>AASEDEFLRYLWRDYLYPKQYAWVLIAAYVAVFVVALVGNTLVCLAVWRNHHMRTVTNYFLVNLSLADVLATAICLPASLLVDITESWLFGHALCKVIPYLQAVSVSVAVLTLSFIALDRWYAICHPLLFKSTARRALGSILGIWAVSLAIMVPQAAVMECSSVLPELAARTRAFSVCDERWADDLAPKIYHSCFFIVTYLAPLGLMAMAYFQIFRKLWGRQIPGTTSALVRNWKRPSDQLGDLEQGLSGEPQPRARAFLAEVKQ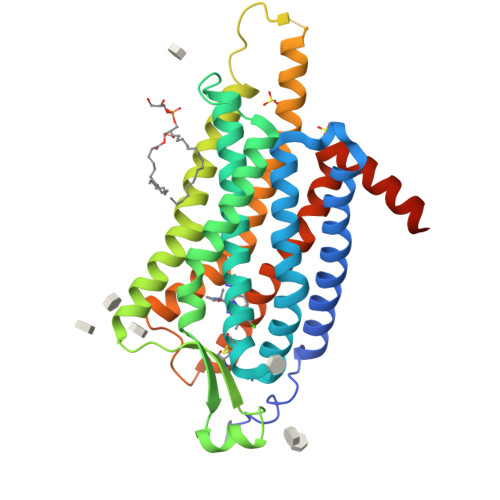MRARRKTAKMLMVVVLVFALCYLPISVLNVLKRVFGMFRQASDREAVYAAFTFSHWLVYANSAANPIIYNFLSGKFREQFKAAFSWWLPGLAAAHHHHHHHHH[2x]N~2~-{4-[4-(4-aminophenyl)buta-1,3-diyn-1-yl]benzoyl}-N-hydroxy-L-isoleucinamide | C23 H23 N3 O3 | 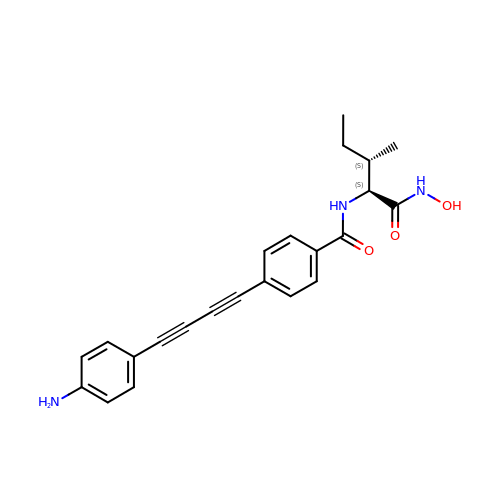VXAKHKNOBREFCR-KKSFZXQISA-N>[4x]GSVDSIREGFQKRCLPVMVLKAKKPFTFETQEGKQEMFHATVATEKEFFFVKVFNTLLKDKFIPKRIIII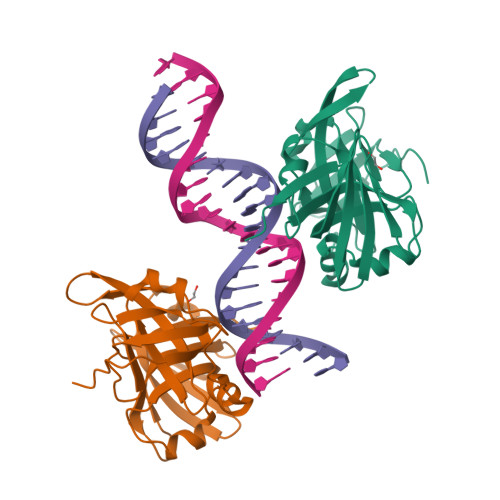ARYYRHSGFLEVNSASRVLDAESDQKVNVPLNIIRKAGETPKINTLQTQPLGTIVNGLFVVQKVTEKKKNILFDLSDNTGKMEVLGVRNEDTMKCKEGDKVRLTFFTLSKNGEKLQLTSGVHSTIKVIKAKKKTAAAS Stalled ribosomes at the endoplasmic reticulum (ER) are covalently modified with the ubiquitin-like protein UFM1 on the 60S ribosomal subunit protein RPL26 (also known as uL24). In a pathway analogous to ubiquitin and other UBLs, post-translational attachment of UFM1 to the lysine residues of target proteins, UFMylation, is catalysed by an enzymatic cascade of E1 (UBA5), E2 (UFC1) and E3 (UFL1) enzymes. Collectively, we identify a fundamental role for UREL in dissociating 60S subunits from the SEC61 translocon and the basis for UFMylation in regulating protein homeostasis at the ER.

We determined the crystal structure of a minimal region of UFL1–UFBP1 that is stable and catalytically competent (E3mUU(ΔUFIM)) in a complex with UFC1. Comparison of the cryo-EM and crystal structure shows that UFL1 WH1 and WH2 superimpose well with a root mean squared deviation of 0.98 Å. The composite pWH–pWH′ domain and UFBP1 WH1′ show almost identical folds in the two structures. Moreover, the crystal structure reveals an N-terminal helix (α1) of UFL1, which is connected to pWH through a hinge. Importantly, this helix mediates multiple hydrophobic interactions with UFC1 α2. Single point mutations in UFC1 (L32R, I40R) or UFL1 (I8R, F15R, Q19R) designed to disrupt this helical interface abolish complex formation between UFC1 and E3mUU(ΔUFIM) and impact ribosome UFMylation without altering the association between UFL1 and UFBP1 in E3mUU(ΔUFIM). While UFL1 α1 binds to UFC1 in the crystal structure, no clear density is visible for UFL1 α1 in the cryo-EM structure. As the composite pWH–pWH′ domain adopts a similar conformation in our structures, it suggests that the hinge region that connects UFL1 pWH and α1 is flexible and enables UFL1 α1 to adopt multiple conformations to optimally position UFC1–UFM1 for catalysis. In the E3mUU(ΔUFIM)–UFC1 crystal structure, UFC1 Asp50 interacts with Arg265 of the DDRGK motif in UFBP1 WH1′. Although the UFC1(D50A) or UFBP1(R265A) mutations do not disrupt complex formation between UFC1 and E3mUU(ΔUFIM), these mutants impair both aminolysis and ribosome UFMylation.

>[2x]MGHHHHHHENLYFQGMADAWEEIRRLAADFQRAQFAEATQRLSERNCIEIVNKLIAQKQLEVVHTLDGKEYITPAQISKEMRDELHVRGGRVNIVDLQQVINVDLIHIENRIGDIIKSEKHVQLVLGQLIDENYLDRLAEEVNDKLQESGQVTISELCKTYDLPGNFLTQALTQRLGRIISGHIDLDNRGVIFT;>[2x]ETMTEEQSQSFLTEFINYIKQSKVVLLEDLASQVGLRTQDTINRIQDLLAEGTITGVIDDRGKFIYITPEELAAVANFIRQRGRVSIAELAQASNSLIAWGRESPAQAPA;>MADEATRRVVSEIPVLKTNAGPRDRELWVQRLKEEYQSLIRYVENNKNADNDWFRLESNKEGTRWFGKCWYIHDLLKYEFDIEFDIPITYPTTAPEIAVPELDGKTAKMYRGGKIKLTDHFKPLWARNVPKFGLAHLMALGLGPWLAVEIPDLIQKGVIQHKEKCNQG[2x]>PQIKVYGLAEKLNPIKAELSNILHTSLIEVLQISPEKRFHRFFPLDKLDFYYPSDRTDNYLIIEIIMFEGRSVETKKQLLRDIFKKVDEKFGISVYDIEITLFEIPKQNWGIRGIPGDELNLSYKVE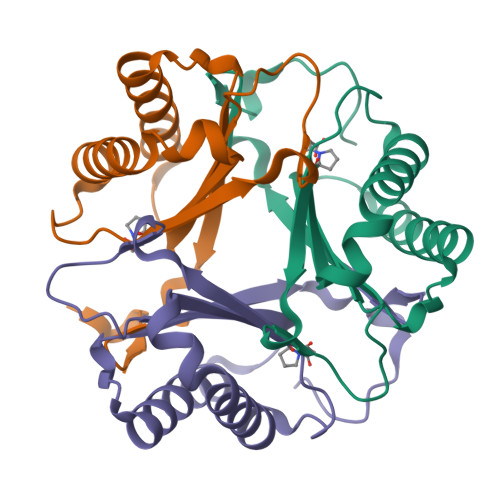V[3x]>[7x]APSLLHKYMGIFFSTMSSEELLGSLDSFDAREDDIFLVSYPKSGTHWLAEVIERIPDAGITLTSPIELGDISKFEELKRIPKRRAIPTHLNYEMLPVTVKQKQCKIIYIVRNPKDTAVSMFHYYRDNPNLPSTETWAAFLELFLKGDVVYGSWFDHVLSWEEHKNDKNVLFIFYEEMKKDFVKSLKKITAFLGIDVNDSEMAKIARSTSFSEMKSNAAKENCDPNHVICALTSDRNLVFRKGVVGDWINYFTPKQNRGFDELFTEKMRNSDVGRCLKEYAHSA;> AILHKYMGIFFSTMSSEELLGSLDSFDAREDDIFLVSYPKSGTHWLAEVIERIPDAGITLTSPIELGDISKFEELKRIPKRRAIPTHLNYEMLPVTVKQKQCKIIYIVRNPKDTAVSMFHYYRDNPNLPSTETWAAFLELFLKGDVVYGSWFDHVLSWEEHKNDKNVLFIFYEEMKKDFVKSLKKITAFLGIDVNDSEMAKIARSTSFSEMKSNAAKENCDPNHVICALTSDRNLVFRKGVVGDWINYFTPKQNRGFDELFTEKMRNSDVGRCLKEYAHSA;>[4x]PSLLHKYMGIFFSTMSSEELLGSLDSFDAREDDIFLVSYPKSGTHWLAEVIERIPDAGITLTSPIELGDISKFEELKRIPKRRAIPTHLNYEMLPVTVKQKQCKIIYIVRNPKDTAVSMFHYYRDNPNLPSTETWAAFLELFLKGDVVYGSWFDHVLSWEEHKNDKNVLFIFYEEMKKDFVKSLKKITAFLGIDVNDSEMAKIARSTSFSEMKSNAAKENCDPNHVICALTSDRNLVFRKGVVGDWINYFTPKQNRGFDELFTEKMRNSDVGRCLKEYAHSA

Cytosolic sulfotransferases (SULTs) are cytosolic enzymes that catalyze the transfer of sulfonate group to key endogenous compounds, altering the physiological functions of their substrates. Enzymatic assays revealed that SULT7A1 is capable of transferring the sulfonate group from 3′-phosphoadenosine 5′-phosphosulfate to the α-carbon of α,β-unsaturated carbonyl-containing compounds, including cyclopentenone prostaglandins as representative endogenous substrates. Since members of the same SULT gene family generally share at least 45% amino acid sequence identity, the newly cloned mouse SULT was judged to belong to a novel SULT family, SULT7, and designated SULT7A1 rather than SULT6B2, as annotated in the NCBI database. Analysis of the amino acid sequence of this novel SULT7A1 showed that it contains a conserved catalytic residue His94 and the signature sequences, called the 5′-phosphosulfate-binding loop, 3′-phosphate-binding loop, and p-loop, that are responsible for the binding to the sulfonate group donor, PAPS.

Although the overall structure of SULT7A1 with 3′-phosphoadenosine-5′-phosphate (PAP) appeared relatively similar to that of mouse SULT1D1, which catalyzes primarily the sulfonation of phenolic compounds, a unique hydrogen bond formed between His94 and Cys234 is present in the active site. It is noted that the Cys234-containing loop (loop-1) occupies the space for a substrate compound docked into the active site. The Cys234-containing loop, however, is flexible based on the high B-factor number. Although loop-1 and segment-1 of SULT1D1 are the key regions forming the substrate entry gate, the flexible loop-1 of SULT7A1 disrupts the entry gate conserved in the other SULTs. Substrate entry gate was not observed in the SULT7A1 structure, but the flexible loop-1 and α-helix following the alternative segment-1 of SULT7A1 may form a potential substrate entry gate. Deleting Cys234 residue appeared to open the substrate entry gate, connecting to active site, formed by the flexible loop-1. Indeed, the C234A mutated SULT7A1 failed to display sulfonating activity toward 2-cylohexenone and 2-cyclopentenone over a wide range of concentrations (1–1,000 μM) tested. In addition to C234A, H51A and H94A also showed no activity to the substrates tested. These findings imply that upon docking of a substrate, the conformation of Cys234-containig loop may be altered and the substrate reaching the active site may then disrupt the hydrogen bound between Cys234 and His94, thereby gaining access to the co-substrate PAPS. It, therefore, appears that His51, His94, and Cys234 are essential residues for the C-sulfonation of α,β-unsaturated carbonyl groups and are critical to the reaction mechanism.>[4x]PKRGKKGAVAEDGDELRTEPEAKKSKTAAKKNDKEAAGEGPALYEDPPDQKTSPSGKPATLKICSWNVDGLRAWIKKKGLDWVKEEAPDILCLQETKCSENKLPAELQELPGLSHQ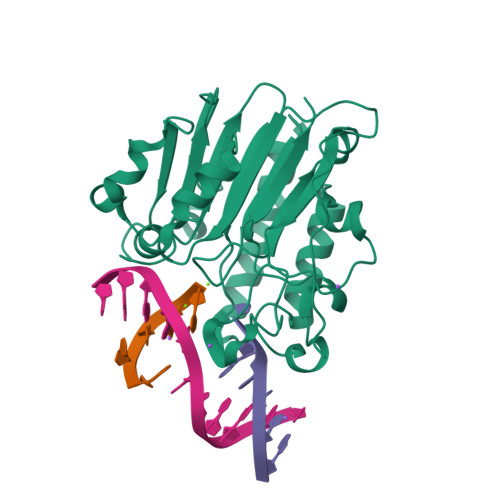YWSAPSDKEGYSGVGLLSRQCPLKVSYGIGDEEHDQEGRVIVAEFDSFVLVTAYVPNAGRGLVRLEYRQRWDEAFRKFLKGLASRKPLVLCGDLNVAHEEIDLRNPKGNKKNAGFTPQERQGFGELLQAVPLADSFRHLYPNTPYAYTFWTYMMNARSKNVGWRLDYFLLSHSLLPALCDSKIRSKALGSDHCPITLYLAL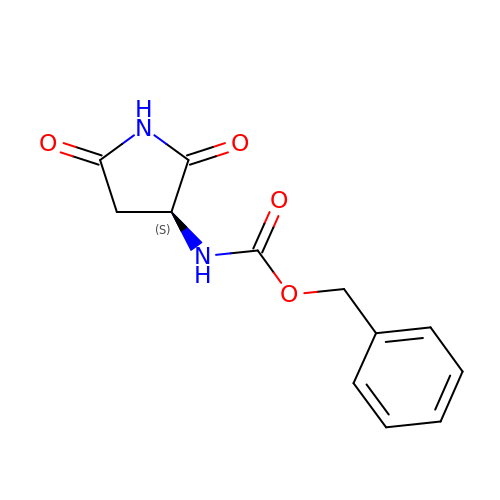(phenylmethyl) ~{N}-[(3~{S})-2,5-bis(oxidanylidene)pyrrolidin-3-yl]carbamate | C12 H12 N2 O4 | QRQMHYISDDHZBY-VIFPVBQESA-N> MTDELKSYEALKAELKKSLQDRREQEDTFDNLQQEIYDKETEYFSHNSNNNHSGHGGAHGSKSHYSGNIIKGFDTFSKSHHSHADSAFNNNDRIFSLSSATYV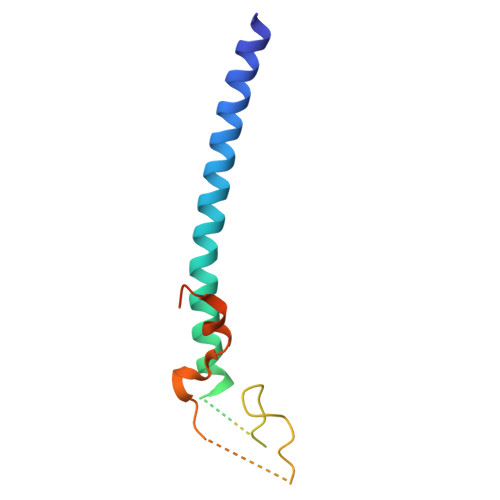KQQHGQSQND>GGSGQPDMSLNVIKMKSSDFLESAELDSGGFGKVSLAFHRTQGLMIMKTVYKGPNCIEHNEALLEEAKMMNRLRHSRVVKLLGVIIEEGKYSLVMEYMEKGNLMHVLKAEMSTPL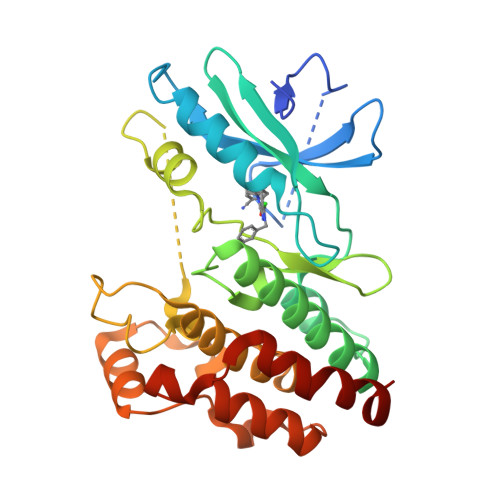SVKGRIILEIIEGMAYLHGKGVIHKDLKPENILVDNDFHIKIADLGLASFKMWSKLNNEEHNELREVDGTAKKNGGTLYYMAPEHLNDVNAKPTEKSDVYSFAVVLWAIFANKEPYENAIAEQQLIMAIKSGNRPDVDDITEYCPREIISLMKLCWEANPEARPTFPGIEEKFRPFYLSQLE[4x]> MKLLHAIQTHAETYPQTDAFRSQGQSLTYQELWEQSDRAAAAIQKRISGEKKSPILVYGHMEPHMIVSFLGSVKAGHPYIPVDLSIPS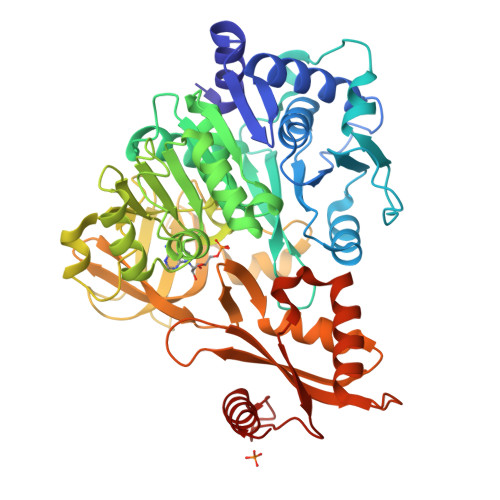ERIAKIIESSGAELLIHAAGLSIDAVGQQIQTVSAEELLENEGGSVSQDQWVKEHETFYIIYTSGSTGNPKGVQISAANLQSFTDWICADFPVSGGKIFLNQAPFSFDLSVMDLYPCLQSGGTLHCVTKDAVNKPKVLFEELKKSGLNVWTSTPSFVQMCLMDPGFSQDLLPHADTFMFCGEVLPVSVAKALLERFPKAKIFNTYGPTEATVAVTSVEITNDVISRSESLPVGFAKPDMNIFIMDEEGQPLPEGEKGEIVIAGPSVSRGYLGEPELTEKAFFSHEGQWAYRTGDAGFIQDGQIFCQGRLDFQIKLHGYRMELEEIEFHVRQSQYVRSAVVIPYQPNGTVEYLIAAIVPEEHEFEKEFQLTSAIKKELAASLPAYMIPRKFIYQDHIQMTANGKIDRKRIGEEVLVRSHHHHHH> GSGDSGSPGRNFNNLTKGLCTINSWHIYGKDNAVRIGESSDVLVTREPYVSCDPDECRFYA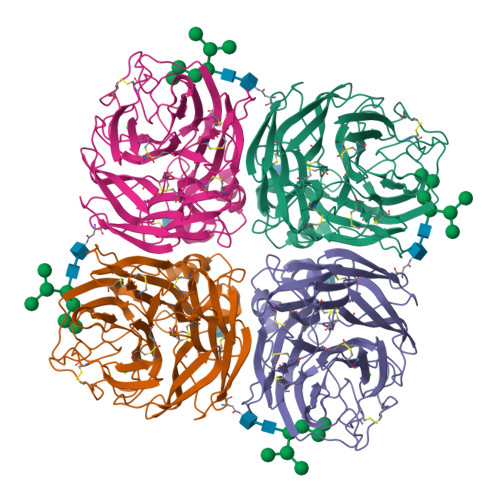LSQGTTIRGKHSNGTIHDRSQYRALISWPLSSPPTVYNSRVECIGWSSTSCHDGKSRMSICISGPNNNASAVVWYNRRPVAEINTWARNILRTQESECVCHNGVCPVVFTDGSATGPADTRIYYFKEGKILKWESLTGTAKHIEECSCYGERTGITCTCRDNWQGSNRPVIQIDPVAMTHTSQYICSPVLTDNPRPNDPNIGKCNDPYPGNNNNGVKGFSYLDGANTWLGRTISTASRSGYEMLKVPNALTDDRSKPIQGQTIVLNADWSGYSGSFMDYWAEGDCYRACFYVELIRGRPKEDKVWWTSNSIVSMCSSTEFLGQWNWPDGAKIEYFL> MNRFVIADSTLCIGCHTCEAACSETHRQHGLQSMPRLRVMLNEKESAPQLCHHCEDAPCAVVCPVNAITRVDGAVQLNESLCVSCKLCGIACPFGAIEFSGSRPLDIPANANTPKAPPAPPAP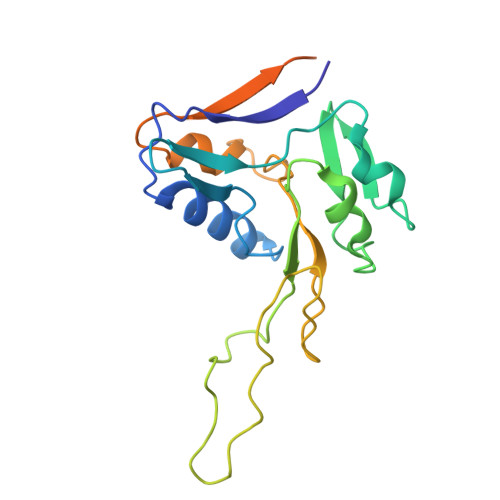ARVSTLLDWVPGIRAIAVKCDLCSFDEQGPACVRMCPTKALHLVDNTDIARVSKRKRELTFNTDFGDLTLFQQAQSGEAK> ADPMIAEELLRAGRLDDALKALQEQVRSQPSNATLRIFLFQLLAVMGQWARAQNQLKVVGELDASALPMVQTYSTAIDCEALRREVFAGRLTPVILGQPAEWIAPLLQALSLDAEGHGEAAQALREQAFDAAPAVPGRIGEAPFAWLADADTRLGPVLEVIVNGRYAWLPMSNLRSLKVEAPSDLRDLVWLPAELTLANGGATVALLPARYAETVEHGDDAARLGRKTEWLDSGLPVGQRLFVTDAGETALFDLRELDFEPTDA

The type VI secretion system (T6SS) is a bacterial nanomachine for the transport of effector molecules into prokaryotic and eukaryotic cells. It involves the assembly of a tubular structure composed of TssB and TssC that is similar to the tail sheath of bacteriophages. The AAA+ ATPase ClpV disassembles the contracted sheath, which resets the systems for reassembly of an extended sheath that is ready to fire again. The interaction of TagJ/HsiE with the sheath as well as with ClpV suggests an alternative mode of disassembly in which HsiE recruits the ATPase to the sheath.

Although HsiE1 (also called TagJ) was found to interact with the essential sheath component HsiB1 (TssB/VipA homolog), its exact role in T6SS remains unclear. Here, we solved the HsiE1 structure from crystals diffracting to 1.2 Å. In the E1-B1 complex structures, there is clear electron density for residues 8–20 of the extraneously added B1 peptide and for residues 8–30 of the co-purified B1 fragment, respectively. Both structures are nearly identical to the structure of HsiE1 alone, with an r.m.s. deviation of 0.4 Å in either case, and to each other with an r.m.s. deviation of 0.3 Å. HsiE1 homologs also show conservation of residues that line the hydrophobic pocket with residues 171 and 181 always tryptophan and proline, respectively, and residue 154 always a large hydrophobic residue (e.g. Phe, Leu, or Trp).>[2x]HHHHHHMRVSFMVAMDENRVIGKDNNLPWRLPSELQYVKKTTMGHPLIMGRKNYEAIGRPLPGRRNIIVTRNEGYHVEGCEVAHSV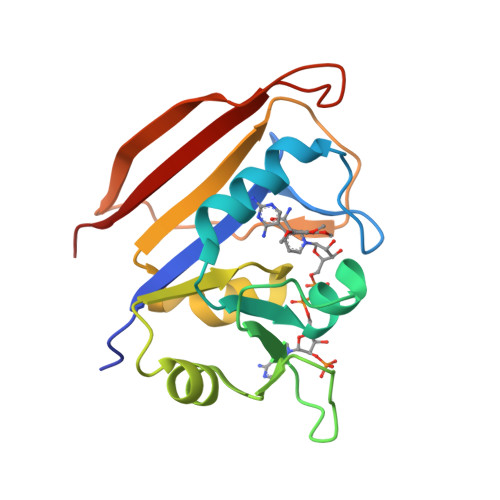EEVFELCKNEEEIFIIGGAQIYDLFLPYVDKLYITKIHHAFEGDTFFPEMDMTNWKEVFVEKGLTDEKNPYTYYYHVYEKQQ>[4x]MKVLFLSADGFEDLE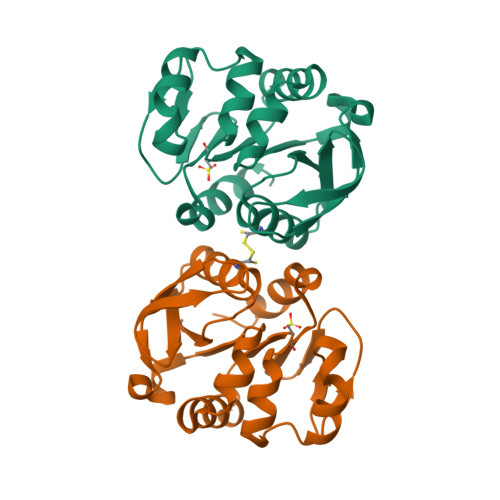LICPLHRIKEEGHEVYVASFERGKITGKHGYSVNVDLAFEEVGPDEFDALVLPGGRAPEIVRLNEKAIEITRKMFEAGKPVASICHGPQILISAGVLKGRKGTSTITIRDDVVNAGAEWVNEEVVVDGNWVSSRHPGDLYAWMREFVKLLK> HHHHHHHHGSGSVPAGAKCRLVETLPENMD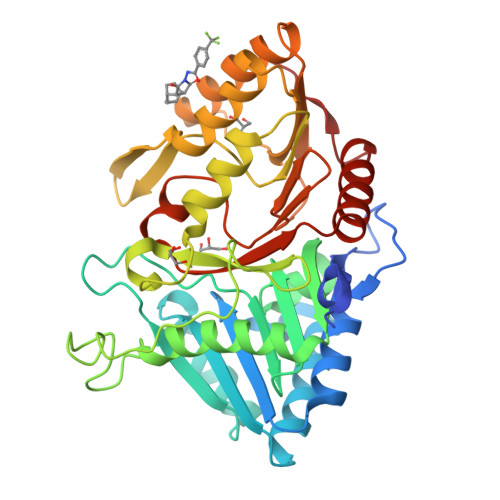FRSDHLTTFECFNEIITLAKKYIYIASFCCNPLSTTRGALIFDKLKEASEKGIKIIVLLDERGKRNLGELQSHCPDINFITVNIDKKNNVGLLLGCFWVSDDERCYVGNASFTGGSIHTIKTLGVYSDYPPLATDLRRRFDTFKAFNSAKNSAANLASAAAALPVSTAYHIKNPIGGVFFTDSPEHLLGYSRDLDTDVVIDKLKSAKTSIDIEHLAIVPTTRVDGNSYYWPDIYNSIIEAAINRGVKIRLLVGNWDKNDVYSMATARSLDELCVQNDLSVKVFTIQNNTKLLIVDDEYVHITSANFDGTHYQNHGFVSFNSIDKQLVSEAKKIFERDWVSSHSKSLKI> MERPWKCCDNIKRLPTKPDPPQWRCNDELEPSQCTAACKSCREAPGPFPGKLICEDIYWGADPGPFCT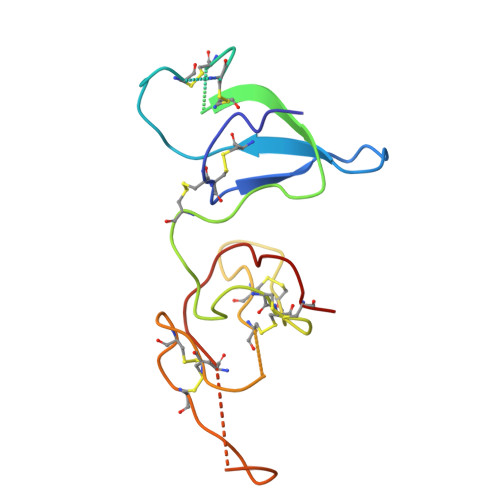PRPWGDCCDKAFCNKMNPPTCRCMDEVKECADACKDCQRVESSEPPRYVCKDRFTGHPGPVCKPR> GSFTNNLEKELLDNFKKNITQYAKQLE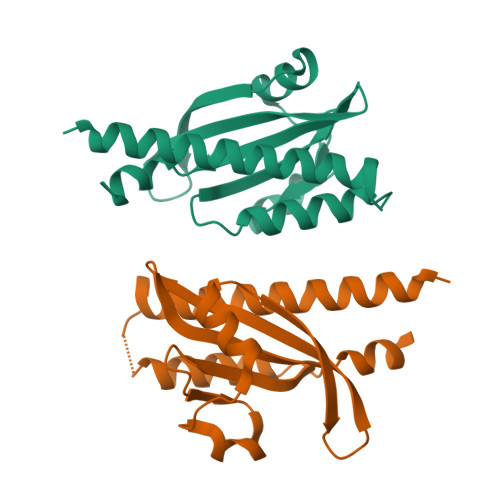ISIEKVYDEKGSVNAQKDIQNLLSEYANRQEIGEIRFIDKDQIIIATTKQSNRSLINQKANDSSVQKALSLGQSNDHLILKDYGGGKDRVWVYNIPVKVDKKVIGNIYIESKINDVYNQLNNINQ>VANPEHYIKHPLQNRWALWFFKNDKSKTWQANLRLISKFDTVEDFWALYNHIQLSSNLMPGCDYSLFKDGIEPMWEDEKNKRGGRWLITLNKQQRRSDLDRFWLETLLCLIGESFDDYSDDVCGAVVNVRAKGD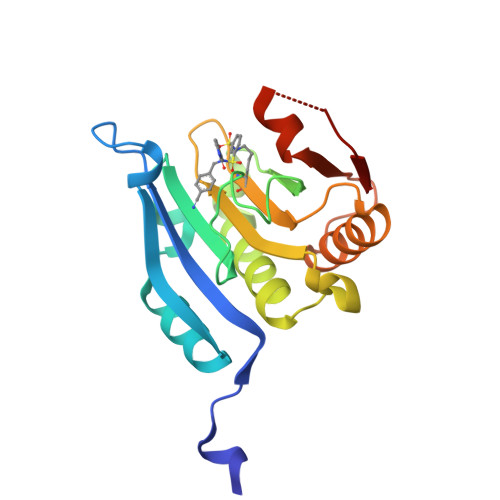KIAIWTTECENRDAVTHIGRVYKERLGLPPKIVIGYQSHADTATKSGSTTKNRFVV[4x]>[2x]MVQQKVEVRLKTGLQARPAALFVQEANRFT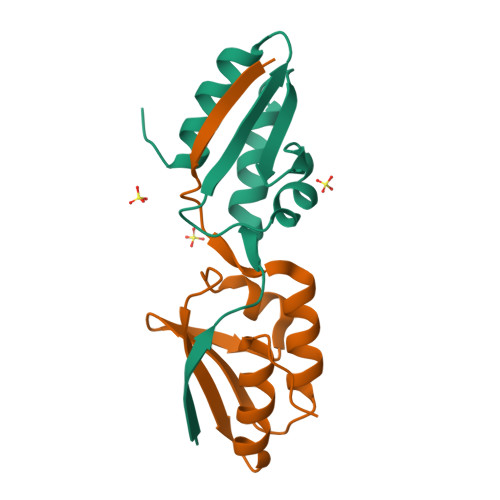SDVFLEKDGKKVNAKSIMGLMSLAVSTGTEVTLIAQGEDEQEALEKLAAYVQEEVLQ> MPYIEKLELKGFKSYGNKKVVIPFSKGFTAIVGANGSGKSNIGDAILFVLGGLSAKAMRASRISDLIFAGSKNEPPAKYAEVAIYFNNEDRGFPIDEDEVVIRRRVYPDGRSSYWLNGRRATRSEILDILTAAMISP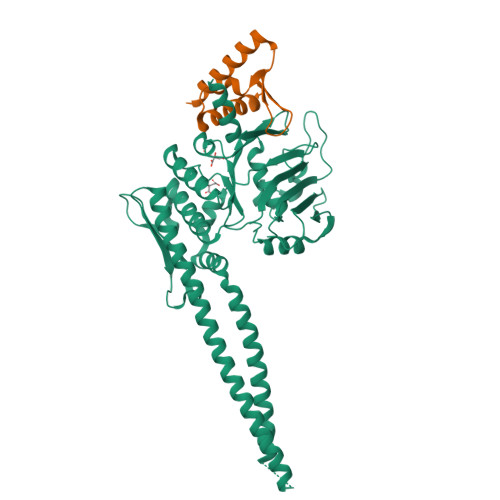DGYNIVLQGDITKFIKMSPLERRLLIDDISGIAEYDSKKEKALEELKQAEENLARVDLLIKEVKSGGSGGSDFEIVERRYLELKSKREKLEAEKESIIEFINEIEKEKKNVFMRTFEAISRNFSEIFAKLSPGGSARLILENPEDPFSGGLEIEAKPAGKDVKRIEAMSGGEKALTALAFVFAIQKFKPAPFYLFDEIDAHLDDANVKRVADLIKESSKESQFIVITLRDVMMANADKIIGVSMRDGVSKVVSLSLEKAMKILEEIRK;> DIEKYVEELYKVVKKIYEKTGTPIKFWDLVPDVEPKIIARTFLYLLFLENMGRVEIIQEEPFGEILVVPMVDKL> MALDVKKYPFIKSLDDELKKYGGGITLTDLLLNSTTLIDQAKDRIQKTKSGDELPHYVSYNEPVLVFYTTLLSLAILNDVKLIRRYAYAEAKQFRSLLHTENEENLLEISKLLDLKINRCDPIKFYLEKKRRIIQKEFCVHFIDYLKYTKDLKEDWKLSGQILHKGYVYLDKNQLIGLIAESIKSKIVEMIRPLNLKEIPEKLKSLIERRGKVEGKFPPQPKKSSDYSWIEKVLEMGLQDSRKRFILYVASRYLVNVKGVNED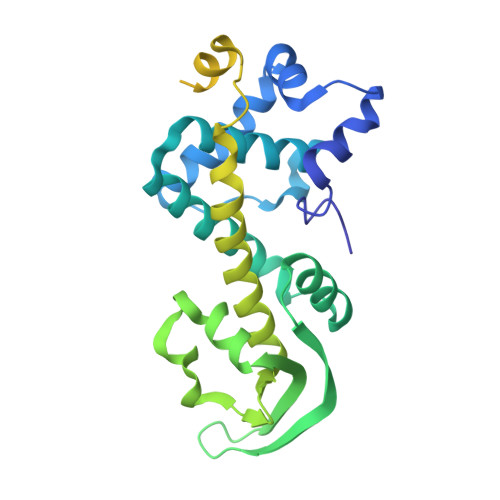EALQTLKEFYYKLQSGKVYESWLKSVINGVKKKGLLPWSLKRIEERDKEMYNEIIRVLKNS> SMTPEQLQAWRWE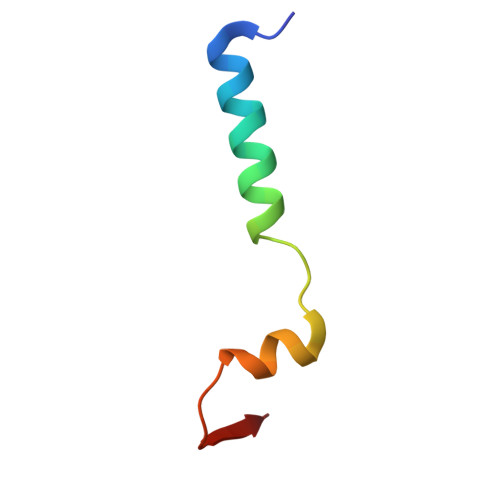REIDERNRPLSDEELDAMFPEGYKVL>GSHMASPAAVNLGTAGNFVILAKSGISTTGTTHVTGDIGVSPITATGMTGFGLTMDSSNTFATSALVTGKAYAADYTPPTPANMSTAVSDMETAYTAAAGVTAPAPVVELGAGNIGGMTLAPGVYKWSTGVTIPTDVTLAGGAND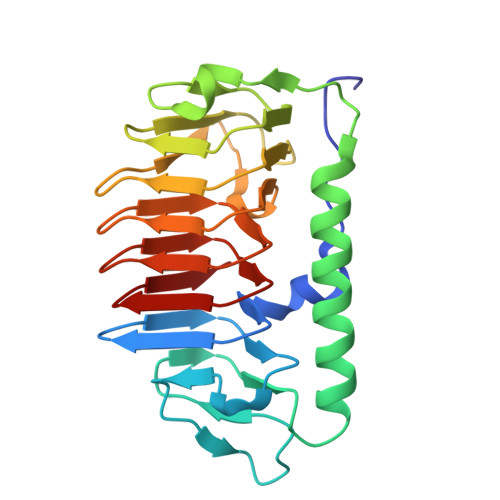VWIFQIAQTLDLSNGIHVNLSGGAQAANIFWQVAGQTTLGTTSVFNGNILDQTAIVLNTGATLNGRALAQTAVTLDASTVSAS[2x]>[3x]GVSLKEDLKDLVRKAEEIGRELSGKLKTNQLRKFHGHLTKIWSNYI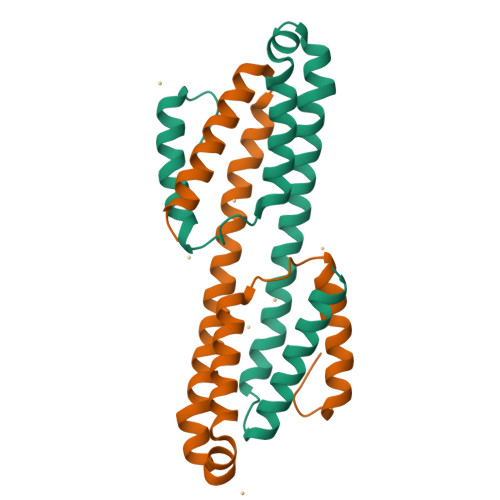YKKKDYRDNPEKFNEEILNELHFMKIFLAYQVGRDIEGISELKEILEPLIDEIKTPDEFEKFKKFYDAILAYHKFHS SpaP is a 1500-residue adhesin expressed on the surface of the caries-implicated bacterium Streptococcus mutans. SpaP is a member of the antigen I/II (AgI/II) family of proteins that are expressed on the surfaces of oral streptococci and are key molecules for networking with other microorganisms and host cells in the oral biofilm. The structure of AgI/II proteins is unique in the sense that the proline-rich region and the alanine-rich region wrap around each other, forming an elongated fibrillar structure that presents the variable domain at the tip. The structure further consists of a C-terminal domain which contains an LPXTG motif that anchors the protein to the cell wall.

The structure of the C-terminal domain of SpaP (residues 1136–1489) was solved and refined to 2.2 Å resolution with six molecules in the asymmetric unit. The final model of SpaP-C1136–1489 from S. mutans consists of six independent protein chains, each binding to two Ca2+ ions. The crystallized protein consists of two domains, C2 and C3, each of which adopts a β-sandwich fold. In each β-­sandwich the two sheets are linked by a covalent isopeptide bond formed between the side chains of a lysine and an asparagine. In the C2 β-sandwich an isopeptide bond is formed between Lys1157 of one sheet and Asn1307 of the other. Similarly, an iso­peptide bond is formed between Lys1334 and Asn1469 of the C3 β-­sandwich. The Ca2+ ions are likely to play important structural roles since they are located in close proximity to the isopeptide bond in each domain. The Ca2+ ion in the C2 domain is coordinated by carboxylate groups from two residues, Asp1208 and Glu1211, the carbonyl O atoms of Lys1261, Tyr1209 and Ala1263 and one water molecule. In C3 the Ca2+ ion is coordinated by side-chain O atoms from Glu1387 and Asp1384, the main-chain O atoms of Lys1430, Gly1431 and Tyr1385 and one water molecule. The overall structure of S. mutans SpaP-C is generally very similar to the structure of S. gordonii SspB-C, with the isopeptide bonds and Ca2+ atoms in identical positions.

>[6x]NYIKPTKVNKNENGVVIDDKTVLAGSTNYYELTWDLDQYKNDRSSADTIQKGFYYVDDYPEEALELRQDLVKITDANGNEVTGVSVDNYTSLEAAPQEIRDVLSKAGIRPKGAFQIFRADNPREFYDTYVKTGIDLKIVSPMVVKKQMGQTGGSYENQAYQIDFGNGYASNIVINNVPKINPKKDVTLTLDPADTNNVDGQTIPLNTVFNYRLIGGIIPANHSEELFEYNFYDDYDQTGDHYTGQYKVFAKVDIILKNGVIIKSGTELTQYTTAEVDTTKGAITIKFKEAFLRSVSIDSAFQAESYIQMKRIAVGTFENTYINTVNGVTYSSNTVKTTT> MGTFTLHQGQTNLIKSFFRNYYLNAELELPKDMELREFALQPFGSDTYVRHLSFSSSEELRDYLVNRNLPLHLFYSSARYQLPSARNMEEKAWMGSDLLFDIDADHLCKLRSIRFCPVCGNAVVSEKCERDNVETLEYVEMTSECIKRGLEQTRNLVEILEDDFGLKPKVYFSGNRGFHVQVDCYGNCALLDSDERKEIAEYVMGIGVPGYPGGSENAPGWVGRKNRGINGVTIDEQVTIDVKRLIRIPNSLHGKSGLIVKRVPNLDDFEFNETLSPFTGYTIFLPYITIETEVLGSIIKLNRGIPIKIKSSIGIYLHLRNLGEVKAYVR;>MALDVKKYPFIKSLDDELKKYGGGITLTDLLLNSTTLIDQAKDRIQKTKSGDELPHYVSYNEPVLVFYTTLLSLAILNDVKLIRRYAYAEAKQFRSLLHTENEENLLEISKLLDLKINRCDPIKFYLEKKRRIIQKEFCVHFIDYLKYTKDLKEDWKLSGQILHKGYVYLDKNQLIGLIAESIKSKIVEMIRPLNLKEIPEKLKSLIERRGKVEGKFPPQPKKSSDYSWIEKVLEMGLQDSRKRFILYVASRYLVNVKGVNEDEALQTLKEFYYKLQSGKVYESWLKSVINGVKKKGLLPWSLKRIEERDKEMYNEIIRVLKNS[2x]

Initiation of DNA synthesis during DNA replication relies on a specialised DNA-dependent RNA polymerase, known as primase. In archaea and eukarya, primase is a constitutive heterodimer of a catalytic subunit, PriS or Pri1, and a regulatory subunit, PriL or Pri27. PriX is required for primase activity and the protein is encoded by a gene that is essential for viability. We have shown that PriX has replaced the Fe–S cluster domain of PriL as the primase module responsible for endowing primase with the ability to initiate nucleic acid synthesis.

To test this hypothesis, we designed and prepared a heterodimeric version of the S. solfataricus primase (named Chimera), which contained wild-type PriS and a second subunit where amino acids 1 to 211 of PriL were fused to amino acids 42 to 154 of PriX, thus excluding the PriL-CTD. Strikingly, Chimera was fully active in primer synthesis assays on both poly(dT) and mixed-sequence DNA templates, in support of the hypothesis that PriX had replaced PriL-CTD as the functional module that cooperates with PriS in S. solfataricus primase. The experiments showed that Chimera was able to prime levels of DNA synthesis that were comparable to those of wild-type PriSLX, thus confirming the results of the primase assay. Interestingly, the crystal structure of Chimera shows that covalently-linked PriX occupies a similar but not identical position relative to PriX in the PriSLX structure, possibly representing an intermediate point in a putative PriX trajectory between initiation and extension states. The cross-linking experiment was performed for both PriSLX and Chimera, yielding equivalent results, in further support of Chimera’s recapitulation of the behavior of wild-type PriSLX. Primer initiation assay showed no primer synthesis by the cross-linked Chimera, in support of the view that the PriSLX conformation, as seen in the crystal structure, is not compatible with primer initiation. However, RNA primer extension assays using either NTP or dNTP did show primer elongation, indicating that the crystal structure of PriSLX represents a biochemically active and potentially physiologically relevant conformation. The fact that the cross-linked Chimera was exclusively active in the extension, but not initiation, of an RNA primer, points to the conformation of the crystal structure as representing a ‘polymerase’ mode. Our evidence of a functional replacement of PriL-CTD by PriX indicates that neither the presence of a Fe–S cluster nor, therefore, its putative redox activity are required for primer synthesis in the archaeal primase of S. solfataricus.Spermidine/spermine N-acetyltransferases (SSATs) are catabolic enzymes that acetylate polyamines and are critical for maintaining intracellular polyamine homeostasis. SpeG is an SSAT protein found in a variety of bacteria, including the human pathogen Vibrio cholerae. This protein adopts a dodecameric structure and contains an allosteric site, making it unique compared to other SSATs. The allosteric site is located between monomers that form the hexamers of the dodecamer, and some evidence has been provided that shows when polyamine binds to these sites, the dodecamer tightens.

Our analysis of the spm-bound structure of VcSpeG showed these two regions form potentially significant contacts: π-π interactions between F32 and F149 and an H-bond between R25 and N152. To elucidate whether these residues could be important for stabilizing the interaction between these two regions of VcSpeG, we created three point mutants: N152L, F149A, and F149G (R3C4-R3C6). We substituted leucine for asparagine at position 152 to retain the overall structural similarity of the residue but remove the ability to H-bond, and we substituted alanine and glycine for phenylalanine at position 149 to potentially decrease the ability of this residue to form hydrophobic interactions. During our kinetic analyses we found the VcSpeG N152L (R3C4), F149A (R3C5), and F149G (R3C6) mutant enzymes still retained reasonably high activity toward spm. The catalytic efficiency of the N152L mutant increased slightly (1.2-fold), and the F149A and F149G mutants decreased 1.4- and 5.3-fold, respectively compared to WT. Our analysis of the spm-bound homology models for the R3C4-R3C6 constructs showed all three retained spm in the allosteric site. Based on these models, a substitution of leucine for asparagine at position 152 (R3C4) caused the H-bond between side chains of R25 and N152 to be disrupted, while the π-π interactions between F32 and F149 side chains were retained. The single point mutants we tested in Region 3 (F149, N152; R3C4-R3C6) were insufficient to totally inhibit enzyme activity. In cases where only a single residue in this region was altered (R3C4-R3C6), the disruption to the activity was far less.

>MNSQLTLRALERGDLRFIHNLNNNRNIMSYWFEEPYESFDELEELYNKHIHDNAERRFVVEDAQKNLIGLVELIEINYIHRSAEFQIIIAPEHQGKGFARTLINRALDYSFTILNLHKIYLHVAVENPKAVHLYEECGFVEEGHLVEEFFILGRYQDVKRMYILQSKYLNRSE[3x]>SKSDVFHLGLTKNDLQGAQLAIVPGDPERVEKIAALMDKPVKLASHREFTSWRAELDGKAVIVCSTGIGGPSTSIAVEELAQLGIRTFLRIGTTGAIQPHINVGDVLVTTASVRLDGASLHFAPMEFPAVADFACTTALVEAAKSIGATTHVGVTASSDTFYPGQERYDTYSGRV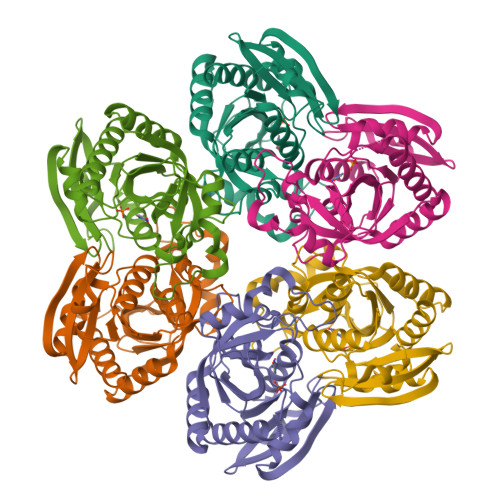VRRFKGSMEEWQAMGVMNYEMESATLLTMCASQGLRAGMVAGVIVNRTQQEIPNAETMKQTESHAVKIVVEAARRLL[6x]>[2x]GPPILKELENLSPEEAAHQKAVVETLLQEDPWRVAKMVKSYLQQHNIPQREVVDTTGLNQSHLSQHLNKGTPMKTQKRAALYTWYVRKQREVAQQ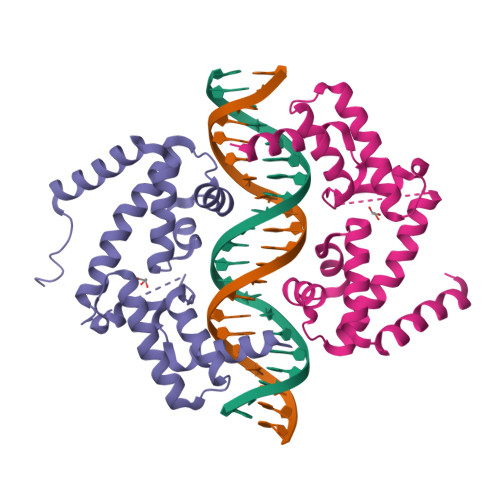FTHAGQGGLIEEPTGDELPTKKGRRNRFKWGPASQQILFQAYERQKNPSKEERETLVEECNRAECIQRGVSPSQAQGLGSNLVTEVRVYNWFANRRKEEAFRH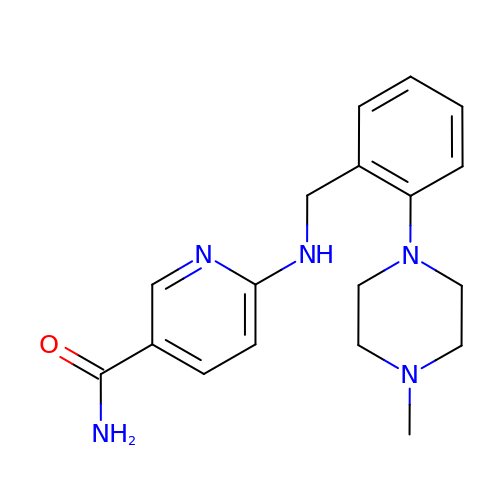6-{[2-(4-methylpiperazin-1-yl)benzyl]amino}pyridine-3-carboxamide | C18 H23 N5 O | BWXGFROIENPTFW-UHFFFAOYSA-N Here we characterize a metal-dependent, bifunctional isoprenyl diphosphate synthase from the leaf beetle Phaedon cochleariae by structural and functional analyses. Isoprenyl diphosphate synthase in P. cochleariae (PcIDS1, EC 2.5.1.1) produces FPP in the presence of Mg2+, but preferably forms GPP when exposed to the heavy metal ions (HMIs) Co2+ or Mn2+. Inter- and intramolecular cooperative effects in the homodimer strongly depend on the provided metal ions and regulate the biosynthetic flux of terpene precursors to either biological defence or physiological development. Strikingly, a unique chain length determination domain adapts to form geranyl or farnesyl pyrophosphate by altering enzyme symmetry and ligand affinity between both subunits.

To obtain a symmetric complex with IPPHAl in both subunits, a strong ligand for the Al site like ZOL is required. This inhibitor significantly increases the thermal stability of all PcIDS1 variants apart from D319A, which prevents coordination of Mg2+B. The protonated imidazole group of ZOLAl imitates the nascent carbocation of DMAPPAl, while the central hydroxymethyl group constrains the bisphosphonate to a fixed conformation. With four negative charges, bisphosphonate resembles the eclipsed PPAl moiety and engages with all metal sites to induce IPPHAl binding in its native orientation. Thus, the binding strength of C5 ligands at the Al site correlates with the affinity for IPPHAl and promotes catalysis in both subunits. However, the enforced closed state through ZOLAl coordination does not provide information about the metal-dependent interplay between the Al and HAl sites.

>[2x]GSFSKEESREFMAIFPDIVRDLTDAGRHTDIPEVTKRFAKVLQYNVPTGKKTRGLSTVIAYKMLEKPENLTPENVRLAGILGWCVELLQASLLIMDDLMDRSETRRGQPCWYRQENVGFLAINDCLHVESSLYSVLRKYFSHLPCYVPIIELFHDVNFKTNMGQSLDALCMKDGRPILSQFTMKRYSSIVKYKTSYYTFQLPVSLGMYLADMYDPEQHRQAKTILMEIGEFFQIQDDFLDAFGDSQVTGKVGTDIKEGKCSWLAVVALQRSNPAQRQIMEEHYGRPEPESTQIIKNLYIELGLPATFAVYEEESFNIIRTHIHQISKGLPHDLFFKIMKKIYKRDA>AMADYDTYVSNVQINNLSYGVYTSGGKETQFFCIGLKHGSEAISINAMCKVDVYGNHKQGFDNMLNTAKYYYTTGGDVRIYYKENVWRDPDFKSAFSSRELIAITTCSSSSYCMGPTVTN[5x];> NISDYKVMTWNLQGSSASTESKWNVNVRQLLSGTAGVDILMVQEAGAVPTSAVPTGRHIQPFGVGIPIDEYTWNLGTTSRQDIRYIYHSAIDVGARRVNLAIVSRQRADNVYVLRPTTVASRPVIGIGLGNDVFLTAHALASGGPDAAAIVRVTINFFRQPQMRHLSWFLAGDFNRSPDRLENDLMTEHLERVVAVLAPTEPTQIGGGILDYGVIVDRAPYSQRVEALRNPQLASDHYPVAFLARSCL;> VDFVYRVDSTPPDVIFRDGFSLLGYNRNFQQFISGRSCSGGSSDSRYIATTSSVNQTYAIARAYYSRSTFKGNLYRYQIRADNNFYSLLPSITYLETQGGHFNAYEKTMMRLQREYVSTLSILPENIQKAVALVYDSATGLVKDGVSTMNASYLGLSTTSNPGVIPFLPEPQTYTQQRIDAFGPLISSCFSIGSVCHSHRGQRADVYNMSFYDARPVIELILSK

Typhoid toxin is an A2B5 protein toxin and an important virulence factor for the human-adapted bacterial pathogen Salmonella enterica serovar Typhi, the causative agent of typhoid fever. Typhoid toxin contains two enzymatic subunits, PltA and CdtB, which dock onto a pentameric delivery platform composed of the protein PltB. It was recently reported that the same enzymatic subunits can assemble with a different delivery platform composed of the protein PltC, forming a distinct version of typhoid toxin. Here, we determined atomic-level structures of the pentameric PltC subunit, the fully assembled PltC typhoid toxin, and the PltC pentamers in complex with glycan receptors.

To gain insight into the structural basis for the organization of PltC typhoid toxin, we determined the crystal structure of PltC-PltA-CdtB holotoxin at 2.29 Å resolution. Similar to the PltB typhoid toxin, PltC typhoid toxin also displays a pyramid-shaped architecture with the PltC homopentamer at the bottom and the two A subunits (CdtB-PltA) sitting on top. As in the PltB typhoid toxin, CdtB does not directly interact with the delivery platform and is tethered to the toxin primarily through the disulfide bond it forms with PltA. Interestingly, the PltA and CdtB subunits sit atop the delivery platform in a nearly identical fashion in both typhoid toxins; PltA and CdtB align with an RMSD of 0.292 Å over 383 Cα atoms in the structures of the two typhoid toxins. Despite the fact that PltC and PltB share very little sequence identity, their interactions with PltA are strikingly similar. In line with the global structural similarities of the PltC and PltB toxin, the C-terminal helix of PltA is inserted into the central pore in a manner that is overall similar in both typhoid toxins. Notably, the pore radius of the channel at the center of the PltC pentamer is generally narrower than that of the PltB pore. Close inspection of the side chain interactions between the PltA C-terminal tail and two different B subunit channels shows that all five monomers from the PltC pentamer interact with the PltA C-terminal tail via 9 direct or water-mediated hydrogen bonds. The charge distribution of the PltC and PltB channels is also very different in the upper part of the pore, the main region that interacts with the C-terminal α-helix of PltA; this region is highly positively charged in PltC and is more hydrophobic in PltB. However, a similar experiment wherein purified PltB toxin (CdtB-His6) was mixed with purified PltC-Strep pentamer showed significant displacement of PltB from PltB toxin by PltC at a 10:1 molar ratio. Together, these results show that PltC’s narrower pore and the stronger electrostatic interactions between this pore and the C-terminal helix of PltA enable PltC to outcompete PltB for assembling typhoid toxin.>[4x]CGCNAAUU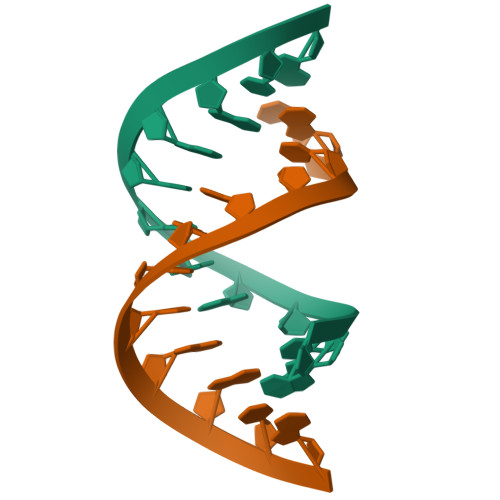GGCG>MGSSHHHHHHSSGRENLYFQGHMPDPAAPGTLRPGGRTARIREAVLLAAGDALAADGFDALDLGEIARRAGVGKTTVYRRWGTPGGLAADLLADMAEQSLPRADTGALEEDLRANARLVVRTLDDPRQGRLFRALIAASLCNEQAA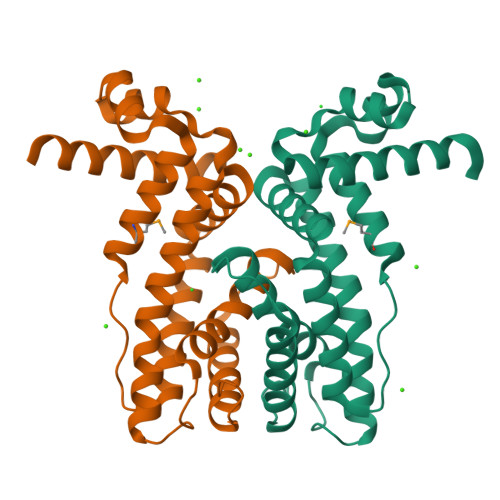EALHRFYAVRVDEWAGCVRDAVARGEVPDGTDPHGVVAAVSAPLYYALLNTGRSLTEADADRAARAASTAARAGVWVTG[2x]> GMTQQTDLQSKTNIDPLAMNDSFLAAADALAVDPMFGIPANVREVIARRGNATRLVILGTKGFGAHLMNVRHERPCEVIAAVDDFRYHSGELYYGLPIISTDRFTELATHDRDLVALNTCRYDGPKRFFDQICRTHGIPHLNFEQAVRAFGLQGNVDYRVDDWGADIVRNIPAFQTLAQRLADDYSVQTLYAVLNFHLTCEPEYYHEVERPYSTLYFRSGLLRFSDSEKMVDCGASIGESLAGLIGVTKGKFERVWMIEPDRINLQTLQNVLRRYTDTNFASRITVHGCGAGENTIRVPFNHEGGHGGFVKPADADHEPADLIDVRPIDDIIDDAPTFIKMDIEGSELSALKGARRAISEHKPKLAISAYHRSTDLLDLTNYI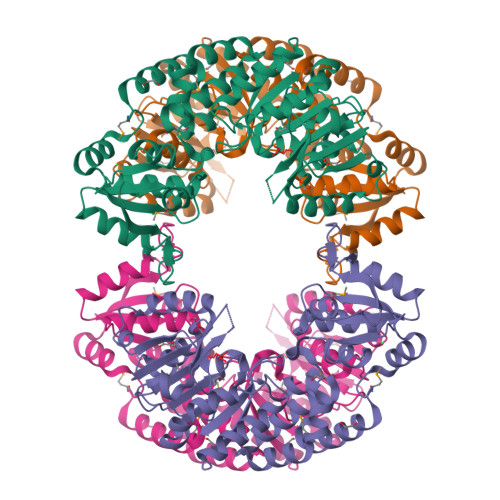LSIRPDYQIGLRHHTPDRWDTCLYFY>ILGGREAEAHARPYMASVQLNGAHLCGGVLVAEQWVLSAAHCLEDAADGKVQVLLGAHSLSQPEPSKRLYDVLRAVPHPDSQPDTIDHDLLLLQLSEKATLGPAVRPLPWQRVDRDVAPGTLCDVAGWGIVNHAGRRPDSLQHVLLPVLDRATCNRRTHHDGAITERLMCAESNRRDSCKGDSGGPLVCGGVLEGVVTSGSAVCGNRKKPGIYTRVASYAAWIDSVLA[2x]

Human factor D (FD) is a self-inhibited thrombin-like serine proteinase that is critical for amplification of the complement immune response. FD is a single-domain serine protease that has a unique physiological substrate. It converts the surface-bound alternative pathway pro-convertase C3bB into the active convertase C3bBb. A salt bridge between Arg202 (Arg218) on the self-inhibitory loop and Asp177 (Asp189) locks the S1 pocket and rigidifies the exosite.

Here, ensemble refinement (ER) of FD and thrombin crystal structures is used to evaluate structure and dynamics simultaneously. Using ER, we detected a highly flexible state of an FD variant [R202A (R218A)]. ER modelled a large number of alternative conformations for the exosite loops, with root-mean-square (r.m.s.) differences in amino-acid positions of up to 6 Å. Different crystal-packing environments of the two copies in the asymmetric unit showed different amounts of disorder of the exosite loops, as indicated by large displacements of the exosite loops 1, 3 and 4 in the first copy and of loop 4 in the other copy. We initially observed an unfolding of the N-terminus that did not account for the observed electron density; therefore, for subsequent runs of this data set a weak harmonic restraint was placed on the Cα atom of the terminal Ile. To assert the consistency of the ensemble model, ten parallel simulations were performed differing only in the random number seed used to generate the initial velocities. The ensemble repeats show high real-space correlation values between ensemble repeats, the majority of which are greater than 0.95, with a minimum of 0.60 around the exosite loops showing high flexibility, demonstrating the reproducibility of the ER method. Release of this conformational interlock results in increased catalytic activity towards artificial peptides and displays a distribution of inactive and active conformations of the catalytic site (60%:40% active:inactive conformations of the catalytic triad, in contrast to the 100% inactive conformation observed in wild-type FD). ER of the FD R202A mutant highlights increased exosite dynamics upon release of the Arg202–Asp177 (Arg218–Asp189) self-inhibitory lock, revealing a highly flexible state reminiscent of an ensemble of conformational states traditionally described as the Na+-free ‘slow’ form of thrombin. The dual role of Arg202 (Arg218) in FD self-inhibition and substrate recognition suggests that the conformational dynamics of the FD R202A (R218A) mutant ensemble may represent a highly flexible intermediate state between the disruption of the Arg202–Asp177 (Arg218–Asp189) self-inhibitory lock and interaction with binding partners.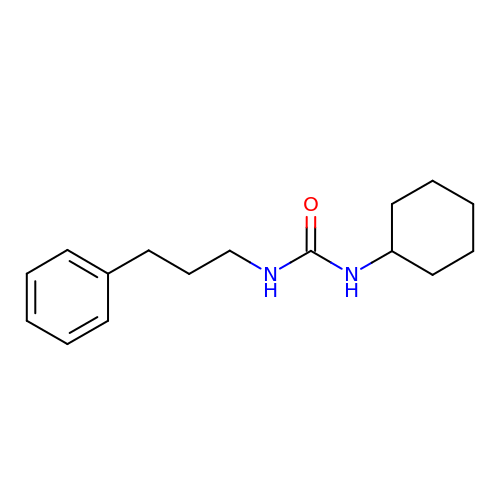N-CYCLOHEXYL-N'-(PROPYL)PHENYL UREA | C16 H24 N2 O | HBTZVNKXMFGOOJ-UHFFFAOYSA-N> PPHGELQYLGQIQHILRCGVRKDDRTGTGTLSVFGMQARYSLRDEFPLLTTKRVFWKGVLEELLWFIKGSTNAKELSSKGVKIWDANGSRDFLDSLGFSTREEGDLGPVYGFQWRHFGAEYRDMESDYSGQGVDQLQRVIDTIKTNPDDRRIIMCAWNPRDLPLMALPPCHALCQFAVV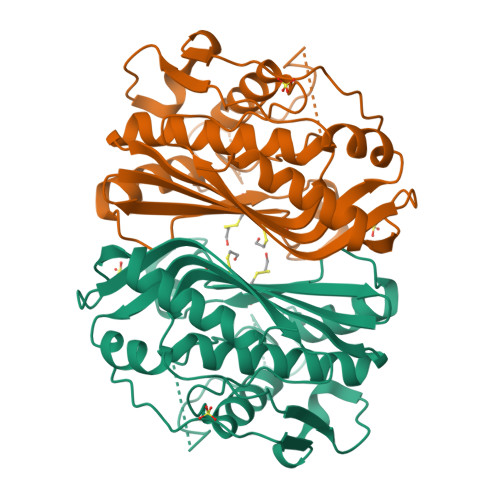NSELSCQLYQRSGDMGLGVPFNIASYALLTYMIAHITGLKPGDFIHTLGDAHIYLNHIEPLKIQLQREPRPFPKLRILRKVEKIDDFKAEDFQIEGYNPHPTIKMEM>GHMSSTNGFGNVYGPSTGTDLFISHSKGVFINGCADCAIYCLPIAGSAFLSNCTNCRVYVACHQLRLKGCTNLDMYVWCASTPIIEECDAMRFGPYRCWVGLLSSCTEDGKTYATHAEWVSRVGEIEDTARTEQNYVKVDDFQWVKKRASPHWCVLAREEERASTTVFGPATLPSSSTAHSTVAADH[2x]

Tubulin-binding cofactor C stimulates GTPase activity and contributes to the release of the heterodimeric α/β-tubulin from a super-complex of tubulin monomers and two ancillary cofactors. There are five TBCs, termed A–E. TBCB and E bind α-tubulin whilst A and D interact with β-tubulin, to deliver each tubulin subunit into a super-complex comprising the α/β-tubulin heterodimer and cofactors D and E. TBCC is involved in the final stage activation of GTP hydrolysis by β-tubulin, promoting release of the α/β-tubulin heterodimer from the super-complex protein assembly that can then proceed to polymerization. This TBCC cofactor is a polypeptide of about 340 amino acids, located in the centrosome and predicted to form three distinct domains.

A recombinant form of this domain, comprising residues 152–355 with a Leu223Met mutation was prepared (LmTBCC-C) to allow the production of selenomethionine (SeMet) derivative protein. The strategy behind the mutation was to enhance the chances of obtaining a good anomalous dispersion signal by placement of selenium into the hydrophobic core of the protein fold at a position unlikely to influence the structure. Two polypeptides constitute the asymmetric unit and in each there are two segments, residues 155–157 and 326–355, which could not be modeled due to disorder. Although previously predicted to consist of two domains the structure is best described as a single domain dominated by a right-handed β-helix of five turns that form a triangular prism. The rest of the polypeptide is catalogued as the TBCC domain but it forms an extended structure, not at all domain-like, mainly positioned over one side of the β-helix, the C-face. There are numerous interactions involving hydrogen bonds and van der Waals forces formed between residues in this extended segment and those on the β-helix, including a tyrosine “ladder” composed of Tyr188, Tyr207 and Tyr224, to stabilize the fold. The structure of the LmTBCC-C domain matches to the human retinitis pigmentosa 2 (RP2) protein with an r.m.s.d. of 2.3 Å and a sequence identity of about 25% over 139 residues. A comparison of the structures is instructive such that we are able to identify, with some confidence, the β-helix A face on LmTBCC-C as the region for interaction with GTP and by implication β-tubulin. In particular LmTBCC Arg214 and Glu234 correspond to RP2 Arg118 and Glu138.>[4x]MGIDTGTSNLVAVEPGAIREDTPAGSVIQYSDYEIDYSSPFAGGVAWIEGEYLPAEDAKISIFDTGFGKSDLTYTVAHVWHGNIFRLGDHLDRLLDGARKLRLDPGYTKDELADITKKCVMLSQLRESFVNLTITRGYGKRPGERDLSKLTNQVYIYAIPYIWAFPPEEQIFGTTAVVPRHVRRAGRNTVDPTIKNYQWGDLTAASFEAKDR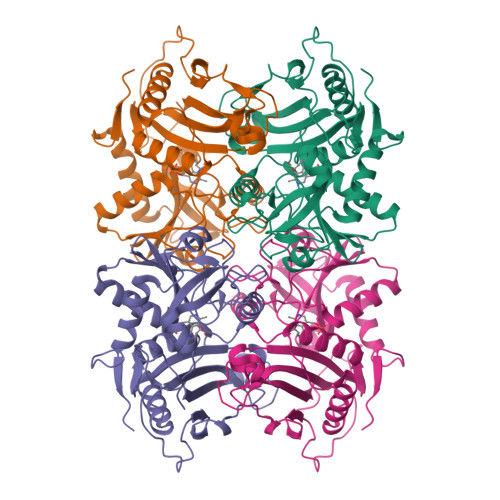GAGTAILMDADNCVAEGPGFNVCIVKDGKLASPSRNALPGITRKTVFEIAGAMGIEAALRDVTSHELYDADEIMAVTTAGGVTPINTLDGVPIGDGEPGPVTVAIRDRFWALMDEPGPLIEAIQY> MFCEKAMELIRELHRAPEGQLPAFNEDGLRQVLEEMKALYEQNQSDVNEAKSGGRSDLIPTIKFRHCSLLRNRRCTVAYLYDRLLRIRALRWEYGSILPNALRFHMAAEEMEWFNNYKRSLATYMRSLGGDEGLDITQDMKPPKSLYIEVR;> MDAAEVEFLAEKELVTIIPNFSLDKIYLIGGDLGPFNPGLPVEVPLWLAINLKQRQKCRLLPPEWMDVEKLEKMRDHERKEETFTPMPSPYYMELTKLLLNHASDNIPKADEIRTLVKDMWDTRIAKLRVSADSFVRQQEAHAKLDNLTLMEINTSGTFLTQALNHMYKLRTNLQPLESTQSQDF;> MSEAYFRVESGALGPEENFLSLDDILMSHEKLPVRTETAMPRLGAFFLERSAGAETDNAVPQGSKLELPLWLAKGLFDNKRRILSVELPKIYQEGWRTVFSADPNVVDLHKMGPHFYGFGSQLLHFDSPENADISQSLLQTFIGRFRRIMDSSQNAYNEDTSALVARLDEMERGLFQTGQKGLNDFQCWEKGQASQITASNLVQNYKKRKFTDMED;> MHHHHHHGRMDYKDDDDKADYKDDDDKADYKDDDDKGRPMTEEVDFLGQDSDGGSEEVVLTPAELIERLEQAWMNEKFAPELLESKPEIVECVMEQLEHMEENLRRAKREDLKVSIHQMEMERIRYVLSSYLRCRLMKIEKFFPHVLEKEKTRPEGEPSSLSPEELAFAREFMANTESYLKNVALKHMPPNLQKVDLFRAVPKPDLDSYVFLRVRERQENILVEPDTDEQRDYVIDLEKGSQHLIRYKTIAPLVASGAVQLI;> MGSHHHHHHG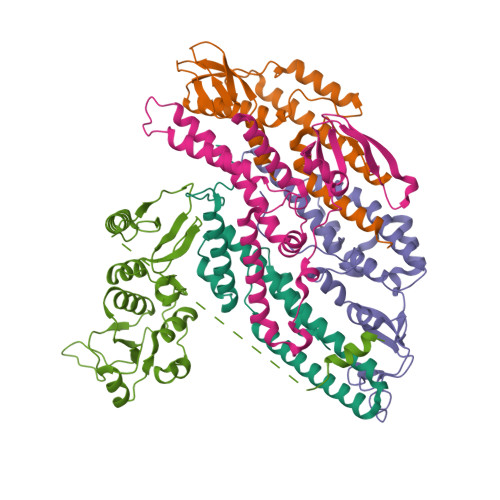SLEVLFQGPHMASNSLNSKLEPTLENLENLDVSAFQAPEDLLDGCRIYLCGFSGRKLDKLRRLINSGGGVRFNQLNEDVTHVIVGDYDDELKQFWNKSAHRPHVVGAKWLLECFSKGYMLSEEPYIHANYQPVEIPVSHQPESKAALLKKKNSSFSKKDFAPSEKHEQADEDLLSQYENGSSTVVEAKTSEARPFNDSTHAEPLNDSTHISLQEENQSSVSHCVPDVSTITEEGLFSQKSFLVLGFSNENESNIANIIKENAGKIMSLLSRTVADYAVVPLLGCEVEATVGEVVTNTWLVTCIDYQTLFDPKSNPLFTPVPVMTGMTPLEDCVISFSQCAGAEKESLTFLANLLGASVQEYFVRKSNAKKGMFASTHLILKERGGSKYEAAKKWNLPAVTIAWLLETARTGKRADESHFLIENSTKEERSLETEITNGINLNSDTAEHPRRAWSHPQFEK> MKVSSPKIQVYSHYPGEYGKENTLICYVSNFHPPDISIELLKNGKVIADAQQTDLAF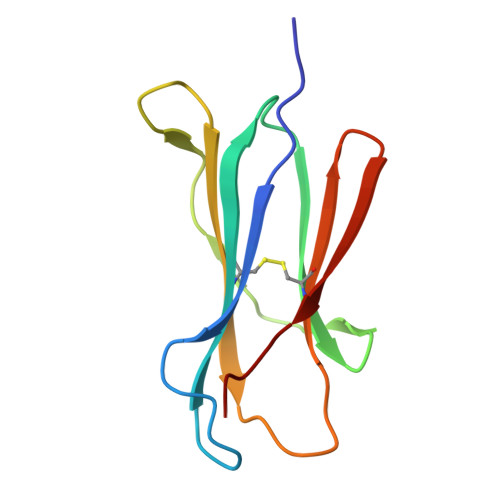EKGWQFHLTKSVSFKPEKSDEYSCRVKHMSDNKTIVWESNM As an essential gene in mammalian development with ubiquitous expression in all eukaryotes, IPMK has important functions at the nexus of many important signaling, metabolic and regulatory pathways, exerting influence through both kinase-dependent and independent roles. The kinase activity of IPMK is a well-characterized node connecting inositol polyphosphate to lipid phosphoinositide signaling, and is critical for AKT activation, Wnt signaling, PLC-mediated IP3/Calcium signaling, nuclear receptor transcriptional activation, mRNA export, and many other roles. All crystal structures of IPK-superfamily kinases have a consensus ATP-grasp fold structurally conserved between family members. However, there are two intrinsically disordered domains in several members of the superfamily: an N-terminal disordered domain and an “internal loop” within the kinase-domain that occurs between S279 and Q373 in human IPMK.

To examine if removal of the two IPMK disordered domains alters IPMK kinetic properties on the PIP2 substrate, the entire disordered N-terminus of human IPMK at D70 with a 6X Histidine tag was replaced, and the kinase-domain internal loop was replaced with a small synthetic Glycine-Serine linker [S279-(GGGGS)2-C373]. Further, removal of the disordered domains from IPMK does not dramatically alter IPMK structure, as a 2.5 Å crystal structure of ΔIPMK maintains all the consensus features of the IPK-superfamily fold. Nevertheless, we were able to solve the structure of human apo-ΔIPMK by molecular replacement using the yeast IPMK as the search model. As with all other members of this superfamily, ΔIPMK has an N-terminal domain consisting of β-sheets 1–3 and α-helix 1, the IP-binding loop consisting of α-helix 2, and a C-terminal domain consisting of the remaining β-sheets 4–7 and α-helices 1, 3, 4, 5 and 6. Two ΔIPMK monomers are in each asymmetric unit of the P21212 space group crystals, with a crystallographic dimerization interface mediated mainly through contacts in the IP-binding helix. We have not observed ΔIPMK to exist as a dimer in size exclusion chromatography, suggesting the dimer in our asymmetric unit is crystallographic. Three of the 6 amino acids of the His-tag in ΔIPMK were weakly ordered in a position next to the β1 strand where nucleotide is predicted to be, if the nucleotide were not lost during cryopreservation. Indeed, ΔIPMK has a KM for ATP of 300 μM, while the ATP KM for wild type IPMK is 61 μM, demonstrating ΔIPMK has a 4.9-fold increased KM for ATP than wild type, despite ΔIPMK having an identical KM and 1.8-fold increased kcat for the PIP2 kinase substrate. Taken together, these crystallographic observations and enzyme kinetic data suggest the native N-terminal sequences of human IPMK can form a previously uncharacterized and structurally conserved ATP clamp, stabilizing ATP binding to IPMK.

>MHHHHHHENLYFQGMDGTVLKQLQPPPRGPRELEFYNMVYAADCFDGVLLELRKYLPKYYGIWSPPTAPNDLYLKLEDVTHKFNKPCIMDVKIGQKSYDPFASSEKIQQQVSKYPLMEEIGFLVLGMRVYHVHSDSYETENQHYGRSLTKETIKDGVSRFFHNGYCLRKDAVAASIQKIEKILQWFENQKQLNFYASSLLFVYEGSSQPTTTKLNDRTLAEKFLSGGGGSGGGGSQEIAEVEVRMIDFAHVFPSNTIDEGYVYGLKHLISVLRSILDN[2x]> XKKKKK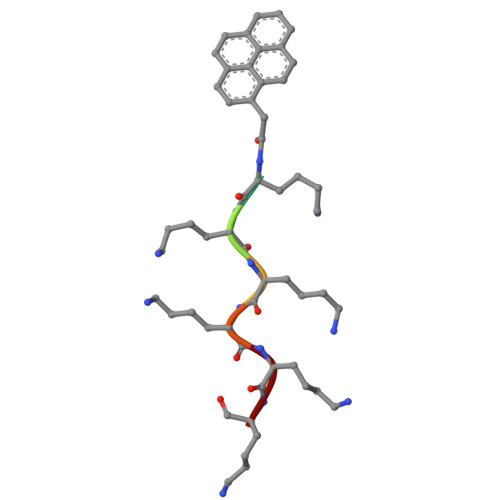K> MGSDKIHHHHHHVLDKIELFILDMDGTFYLDDSLLPGSLEFLETLKEKNKRFVFFTNNSSLGAQDYVRKLRNMGVDVPDDAVVTSGEITAEHMLKRFGRC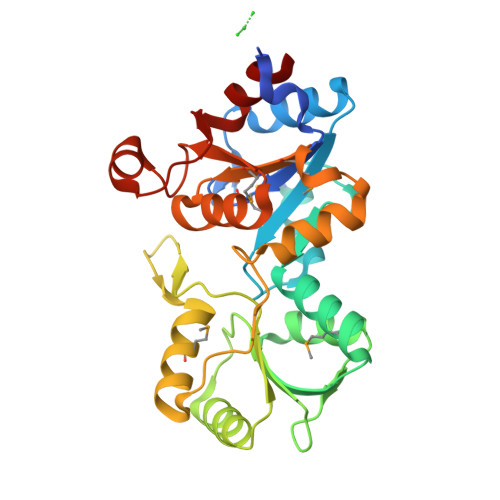RIFLLGTPQLKKVFEAYGHVIDEENPDFVVLGFDKTLTYERLKKACILLRKGKFYIATHPDINCPSKEGPVPDAGSIMAAIEASTGRKPDLIAGKPNPLVVDVISEKFGVPKERMAMVGDRLYTDVKLGKNAGIVSILVLTGETTPEDLERAETKPDFVFKNLGELAKAVQ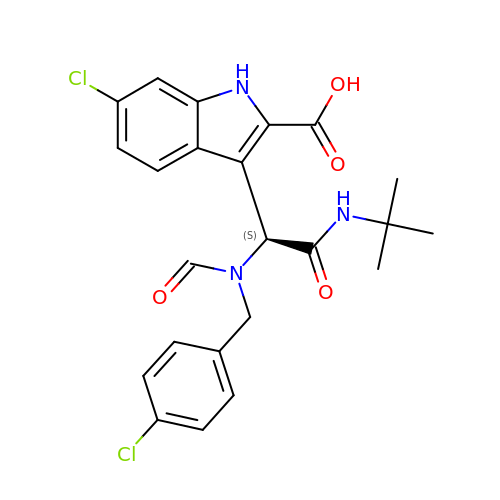3-{(1S)-2-(tert-butylamino)-1-[(4-chlorobenzyl)(formyl)amino]-2-oxoethyl}-6-chloro-1H-indole-2-carboxylic acid | C23 H23 Cl2 N3 O4 | ZAOJHZGIRKVCBH-FQEVSTJZSA-N> SSLPVPYKLPVSLSVGSCVIIKGTPIHSFINGPQLQVDFYTDMDEDSDIAFHFNVRFGNHVVMNRREFGIWMLEETTDYVPFEDGKQFELCIYVHYNEYEIKVNGIRIYGFVHRIPPSFVKMVQVSRDISLTSVCVCN

Galectin (Gal) is a lectin that binds to β-galactosides. Because the primary and tertiary structures of Gal-13 are highly conserved among all galectins, it had been named galectin-13. However, our crystallographic and biochemical experiments (solid phase experiment, hemagglutination assay, and biolayer interferometry) proved that wild-type Gal-13 could not bind lactose or a rhamnogalacturonan Ι domain (RG-I-4) from Ginseng Pectin. Primary structure alignment showed that a highly conserved histidine residue was modified to arginine (Arg53) in the ligand binding site of wild-type Gal-13, which may be why Gal-13 could not bind lactose.

All three other variants (R53HH57R, R53HR55NH57R, and R53HR55NR57RD33G) co-crystallized with lactose, but not Tris, even when the crystallization conditions contained 100 mM Tris. This indicates that these three variants prefer to binding lactose. Without this residue, Gal-13 cannot bind lactose. Moreover, in the crystal, Asp33 from one monomer occupies part of the ligand binding site of another Gal-13 monomer. In order to eliminate steric hindrance, this aspartate was mutated to glycine in several variants. However, the pyran surface of the galactose residue in different structures could not be totally merged with each other, and glucose residues showed variable conformations. The conserved tryptophan and histidine residues in the three variants showed the same conformation and position as in Gal-3 and Gal-8N. In Gal-13 variants, His53, Asn55, and Arg57 in Gal-13 variants show similar conformations to the corresponding residue of Gal-3 CRD and Gal-8 N CRD.> RQLALEAKGETPSAVTRLSVVAKSEPQDEQSRSQSARRIILSRLKAGEVDLLEEELGHLTTLTDVVKGADSLSAILPGDIAEDDITAVLCFVIEADQITFE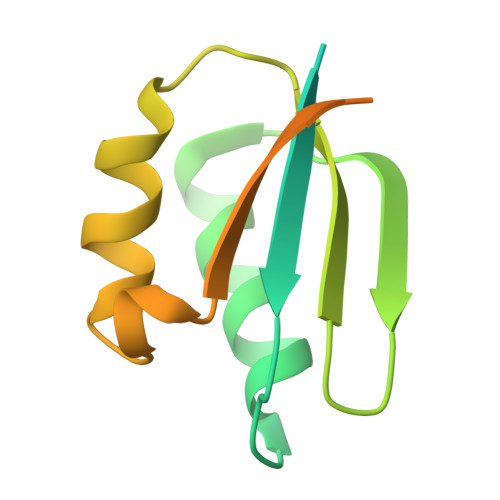TVEVSPKISTPPVLKLAAEQAPTGRVEREKTTR2-[4-[(2~{S})-3-[(6-chloranyl-1-propan-2-yl-benzimidazol-2-yl)amino]-2-oxidanyl-propoxy]phenyl]ethanenitrile | 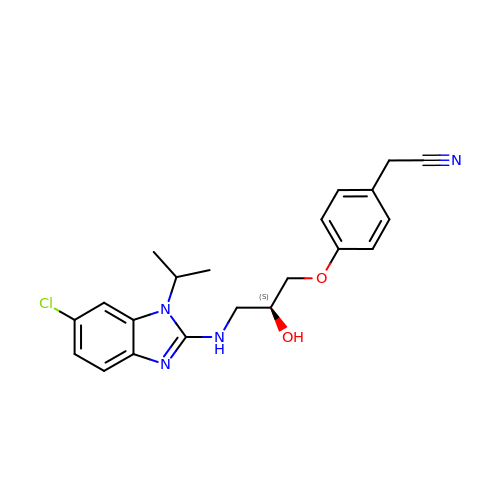C21 H23 Cl N4 O2 | SYDWHCIVWIRKCC-KRWDZBQOSA-N>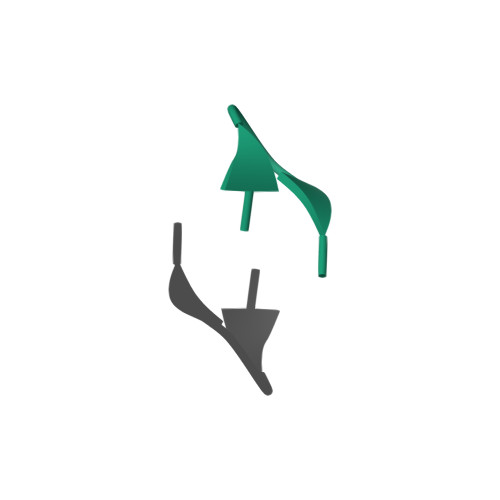 ANKHPEANKHPE{4-[6-BROMO-3-(BUTYLAMINO)IMIDAZO[1,2-A]PYRIDIN-2-YL]PHENOXY}ACETIC ACID | C19 H20 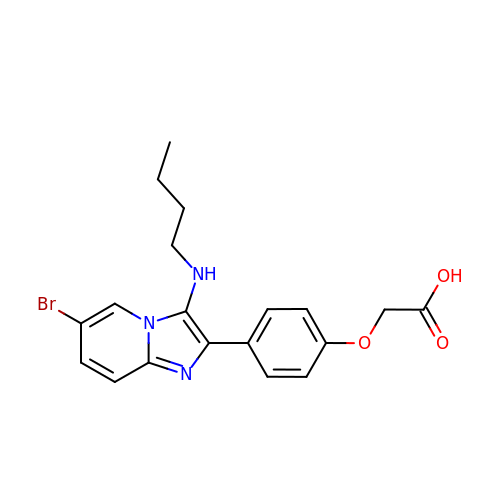Br N3 O3 | OZIYUZINTQIIAN-UHFFFAOYSA-N>[4x]KLCRLCPWDWTFLLGNCYFFSKSQRNWNDAVTACKEVKAQ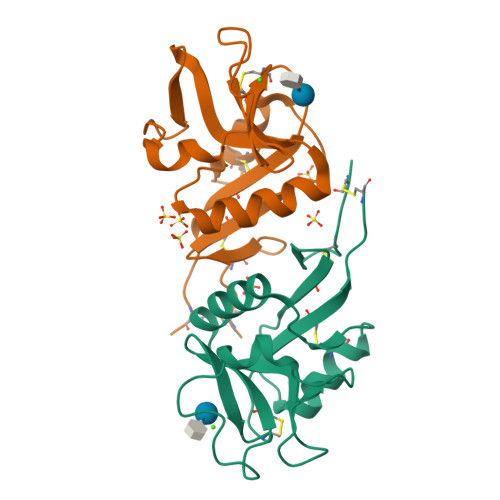LVIINSDEEQTFLQQTSKAKGPTWMGLSDLKKEATWLWVDGSTLSSRFQKYWNRGEPNNIGEEDCVEFAGDGWNDSKCELKKFWICKKSATPCT> LPGECSVNVIPKKNLDKAKFFSGTWYETHYLDMDPQATEKFCFSFAPRESGGTVKEALYHFNVDSKVSFYNTGTGPLESNGAKYTAKFNTVDKKGKEIKPADEKYSYTVTVIEAAKQSALIHICLQEDGKDIGDLYSVLNRNKNALPNKKIKKALNKVSLVLTKFVVTKDLDCKYDDKFLSSW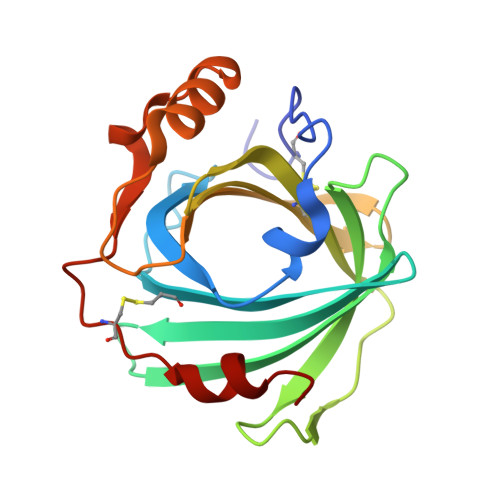QK> MSVLSSVSMGSRIGSSLLGRSSAYLAQCGFSTRSNLNGSIDTSSSVFQALSSDNENKPAASPLNVKLPGMSCSSILLPKTSRIAVPFGNQTMAMSSVRDVKTGSLPTNFLTGVYRFWRSQNPAEKPHDPVNDRLLPAVVD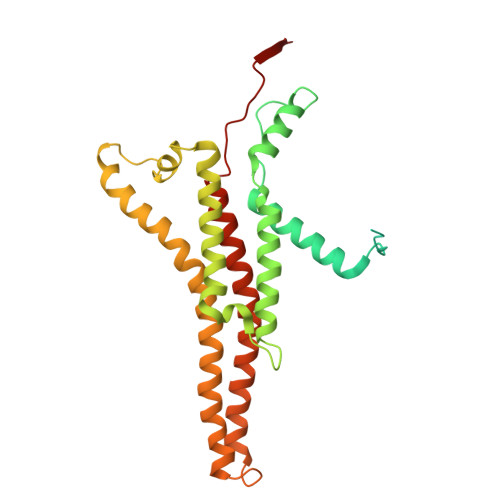ASDKRASIGTWATTFFCTIISCNLLGLMPFNEAPTSGLGFATGLGVSVWATATILGLSKTGFKFPGHFIPGGTPWPMAFIFVPLETISYTFRAVSLGVRLWVNMLAGHTLLHILTGMALALPFSLGFFSMVPATFGVCCLLSALVGLEYLVAVLQSGVFSILSTVYVGEFNHDKFIGPAAKIVKKIH> MGSNQSSSTSTKKLKAGNFDVAYQNPDKAIKGGNLKVAYQSDSPMKAQWLSGLSNDATFATMSGPGGGQDGLFFTDSGFKFIKGGAADVALDKESKTATITLRKDLKWSDGSEVTAKDYEFTYETIANPAYGSDRWTDSLANIVGLSDYHTGKAKTISGITFPDGENGKVIKVQFKEMKPGMTQSGNGYFLETVAPYQYLKDVAPKDLASSPKTTTKPLVTGPFKPENVVAGESIKYVPNPYYWGEKPK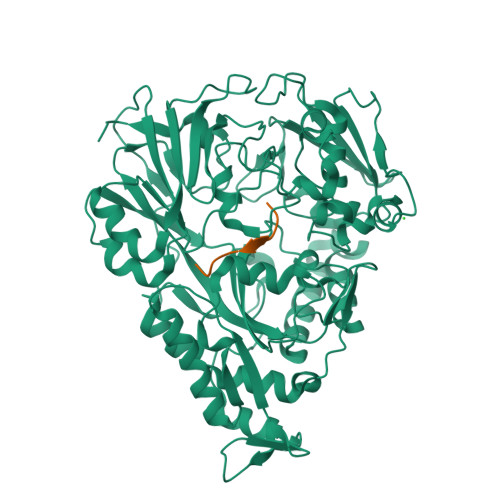LNSITYEVVSTAKSVAALSSSKYDIINGMVSSQYKQVKNLKGYKVLGQQAMYISLMYYNLGHYDAKNSINVQDRKTPLQDQNVRQAIGYARNVAEVDNKFSNGLSTPANSLIPPIFKQFTSSSVKGYEKQDLDKANKLLDEDGWKLNKSTGYREKDGKELSLVYAARVGDANAETIAQNYIQQWKKIGVKVSLYNGKLMEFNSWVDHMTTPPGANDWDITDGSWSLASEPSQQDLFSAAAPYNFGHFNDSEITKDLNDIDSAKSENPTYRKAAFVKYQEDMNKKAYVIPTNFMLNYTPVNKRVVGMTLDYGAMNTWSEIGVSSAKLATKGSIEGRHHHHHH;> RPPGFSPFA> KFSKQSWGLENEALIVRCPRQGKPSYTV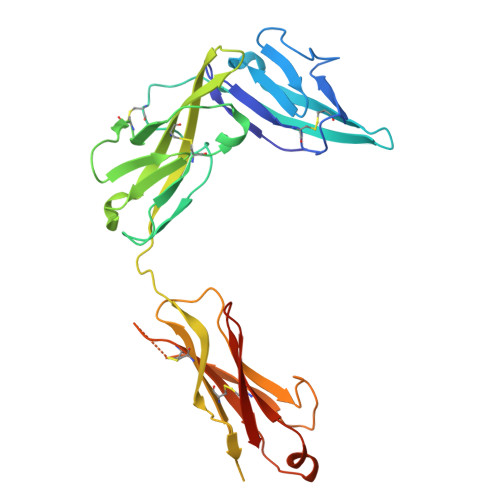DWYYSQTNKSIPTQERNRVFASGQLLKFLPAAVADSGIYTCIVRSPTFNRTGYANVTIYKKQSDCNVPDYLMYSTVSGSEKNSKIYCPTIDLYNWTAPLEWFKNCQALQGSRYRAHKSFLVIDNVMTEDAGDYTCKFIHNENGANYSVTATRSFTVKDEQGFSLFPVIGAPAQNEIKEVEIGKNANLTCSACFGKGTQFLAAVLWQLNGTKITDFGEPRIQQEEGQNQSFSNGLACLDMVLRIADVKEEDLLLQYDCLALNLHGLRRHTVRLSRKHHHHHH>ATTGTQGYTVVKNDWKKAVKQLQDGLKDNSIGKITVSFNDGVVGEVAPKSANKKADRDAAAEKLYNLVNTQLDKLGDGDYVDFSVDYNLENKIITNQADAEAIVTKLNSLNEKTLIDIATKDTFGMVSKTQDSEGKNVAATKALKVKDVATFGLKSGGSEDTGYVVEMKAGAVEDKYGKVGDSTAGIAINLPSTGLEYAGKGTTIDFNKTLKVDVTGGSTPSAVAVSGFVTKDDTDLAKSGTINVRVINAKEESIDIDASSYTSAENLAKRYVFDPDEISEAYKAIVALQNDGIESNLVQLVNGKYQVIFYPEGKRLE[2x];>NDTIASQDTPAKVVIKANKLKDLKDYVDDLKTYNNTYSNVVTVAGEDRIETAIELSSKYYNSDDKNAITDKAVNDIVLVGSTSIVDGLVASPLASEKTAPLLLTSKDKLDSSVKSEIKRVMNLKSDTGINTSKKVYLAGGVNSISKDVENELKNMGLKVTRLSGEDRYETSLAIADEIGLDNDKAFVVGGTGLADAMSIAPVASQLKDGDATPIVVVDGKAKEISDDAKSFLGTSDVDIIGGKNSVSKEIEESIDSATGKTPDRISGDDRQATNAEVLKEDDYFTDGEVVNYFVAKDGSTKEDQLVDALAAAPIAGRFKESPAPIILATDTLSSDQNVAVSKAVPKDGGTNLVQVGKGIASSVINKMKDLLDM[2x]

The surfaces of most bacteria and archaea are covered with a proteinaceous coat, the surface or S-layer, which is formed through the self-assembly of individual protein subunits into a regularly spaced, two-dimensional array. In C. difficile, the S-layer largely consists of a major S-layer protein, SlpA, which assembles into a paracrystalline array enveloping the cell. The major protein of the C. difficile S-layer, SlpA, is post-translationally cleaved into two S-layer proteins (SLPs): the high molecular weight (HMW) and low molecular weight (LMW), herein referred to as SLPH and SLPL, respectively. These subunits then form a complex (referred to as H/L) that is incorporated in the S-layer.

Our H/L structural model reveals three distinct regions: a pseudo-threefold symmetric SLPH tile, an intricate LID/HID interacting motif and a third region composed of two domains, D1 and D2, of SLPL. These regions define two separate planes, with the SLPL spanning ~35 Å above the SLPH plane, linked by the LID/HID motif. The three CWB2 motifs form a triangular prism and adopt an intertwined fold, with a β-strand from one CWB2 inserting into the neighbouring domain to complete a β-sheet (β2H in CWB21 completes CWB23, strand β6H from CWB22 inserts into CWB21 and β10H in CWB23 is inserted into CWB22) sandwiched between two α-helical regions. The environment- and cell-facing sides of SLPH exhibit considerable charge differences, with a mostly negatively charged external surface and a largely non-polar cell wall-facing base, decorated by positive patches. In the crystal, two H/L complexes, related by pseudo-twofold symmetry, are present in the P1 asymmetric unit, packed in a 2D planar array which is then stacked to extend the crystal into the third dimension. The 2D lattice is achieved by tiling of SLPH, with interlocked ridges of SLPL molecules covering gaps between the tiles, creating a tightly packed layer. As hypothesised, the p2 symmetric 2D lattices of native S-layer ghosts (a = b = 80 Å, γ = 100°) were consistent with unit cell parameters of the stacked lattices in the 2D plane of the X-ray crystals (b = 78 Å, c = 80 Å, α = 100°), pointing towards a similar packing. In contrast, tiling of SLPH and the SLPL ridges generate a compact lattice apart from two distinct pores in the C. difficile S-layer array. Pore 1 (cyan arrow, between molecules 1 and 3) is ~20 Å across the widest point at the environment-facing surface but is partially occluded by the LID/HID motif narrowing it down to an 11 Å wide cavity. The second pore, formed between two SLPH (molecules 1 and 2) is fully accessible from both outer and inner surfaces of the layer.>[11x]MAAKVFESIGKFGLALAVAGGVVNSALYNVDAGHRAVIFDRFRGVQDIVVGEGTHFLIPWVQKPIIFDCRSRPRNVPVITGSKDLQNVNITLRILFRPVASQLPRIFTSIGEDYDERVLPSITTEILKSVVARFDAGELITQRELVSRQVSDDLTERAATFGLILDDVSLTHLTFGKEFTEAVEAKQVAQQEAERARFVVEKAEQQKKAAIISAEGDSKAAELIANSLATAGDGLIELRKLEAAEDIAYQLSRSRNITYLPAGQSVLLQLPQLEDYKDHDGDYKDHDIDYKDDDDK;>[11x]MAQNLKDLAGRLPAGPRGMGTALKLLLGAGAVAYGVRESVFTVEGGHRAIFFNRIGGVQQDTILAEGLHFRIPWFQYPIIYDIRARPRKISSPTGSKDLQMVNISLRVLSRPNAQELPSMYQRLGLDYEERVLPSI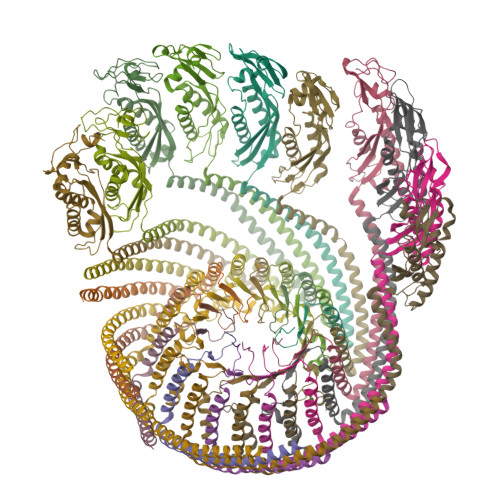VNEVLKSVVAKFNASQLITQRAQVSLLIRRELTERAKDFSLILDDVAITELSFSREYTAAVEAKQVAQQEAQRAQFLVEKAKQEQRQKIVQAEGEAEAAKMLGEALSKNPGYIKLRKIRAAQNISKTIATSQNRIYLTADNLVLNLQDESFTRGSDSLIKGKK> YTFIDYAIEYSEKYAPLRQKLLSTDIGSVASFLLSRESRAITGQTIYVDNGLNIMFLPD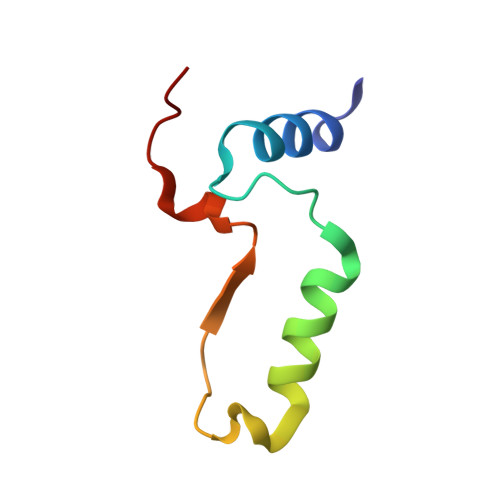D>MSIIVISGCATGIGAATRKVLEAAGHQIVGIDIRDAEVIADLSTAEGRKQAIADVLAKCSKGMDGLVLCAGLGPQTKVLGNVVSVNYFGAT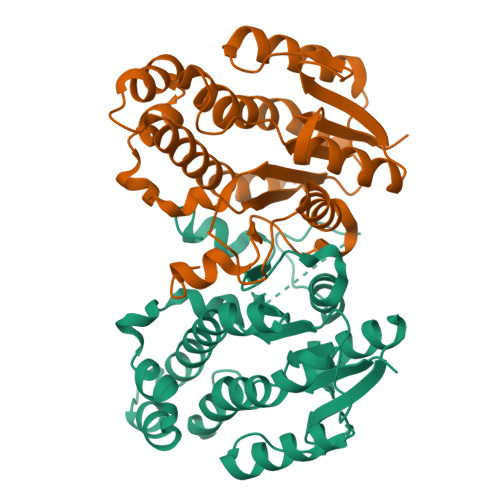ELMDAFLPALKKGHQPAAVVISSVASAHLAFDKNPLALALEAGEEAKARAIVEHAGEQGGNLAYAGSKNALTVAVRKRAAAWGEAGVRLNTIAPGATETPLLQAGLQDPRYGESIAKFVPPMGRRAEPSEMASVIAFLMSPAASYVHGAQIVIDGGIDAVMRPTQF[2x]>SNAGGSSPITGLVYDQRMMLHHNMWDSHHPELPQRISRIFSRHEELRLLSRCHRIPARLATEEELALCHSSKHISIIKSSEHMKPRDLNRLGDEYNSIFISNESYTCALLAAGSCFNSAQAILTGQVR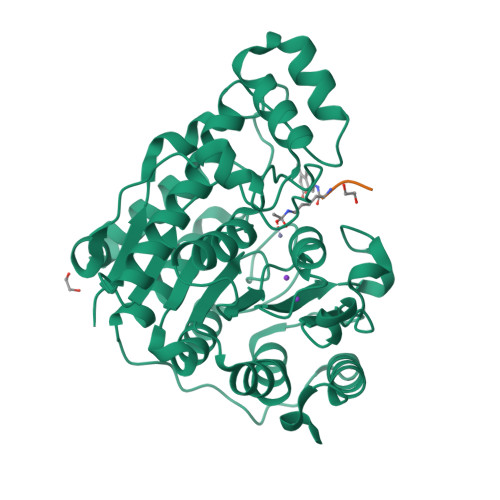NAVAIVRPPGHAAEKDTACGFCFFNTAALTARYAQSITRESLRVLIVDWDVHHGNGTQHIFEEDDSVLYISLHRYEDGAFFPNSEDANYDKVGLGKGRGYNVNIPWNGGKMGDPEYMAAFHHLVMPIAREFAPELVLVSAGFDAARGDPLGGFQVTPEGYAHLTHQLMSLAAGRVLIILEGGYNLTSISESMSMCTSMLLGDSPPSLDHLTPLKTSATVSINNVLRAHAPFWSSLR[2x]> TSPTTTSTGTGTGSSTDQAISPLVEGENAPEVTTAKLGFIALTDAAPLIIAKEKGFYAKYGMPDVEVLKQASWGTTRDNLVLGSASGGIDGAHILTPMPYLITMGTVTDGKPTPMYILARLNVNGQGIQLGNNYKDLKVGTDAAPLKEAFAKVTDPKVAMTFPGGTHDMWIRYWLAAGGMEPGKDFSTIVVPPAQMVANVKVNAMESFCVGEPWPLQTVNQGVGYQALTTGQLWKDHPEKAFGMRADWVDQNPKAAKALLMAVM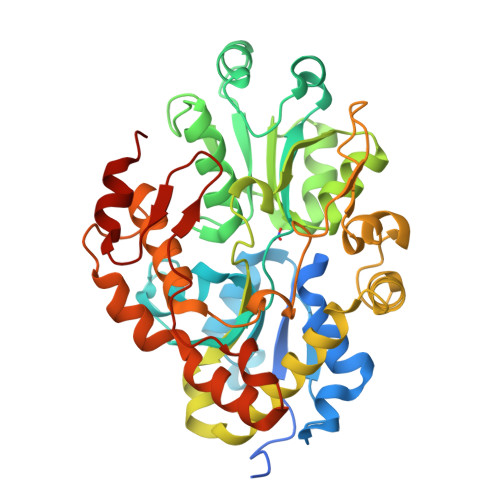EAQQWCDQAENKEEMCQILSKREWFKVPFEDIIDRSKGIYNFGNGQETFEDQEIMQKYWVDNASYPYKSHDQWFLTENIRWGYLPASTDTKAIVDKVNREDLWREAAQALEVPADQIPSSPSRGIETFFDGITFDPENPQAYLDSLKIKSIKA>[2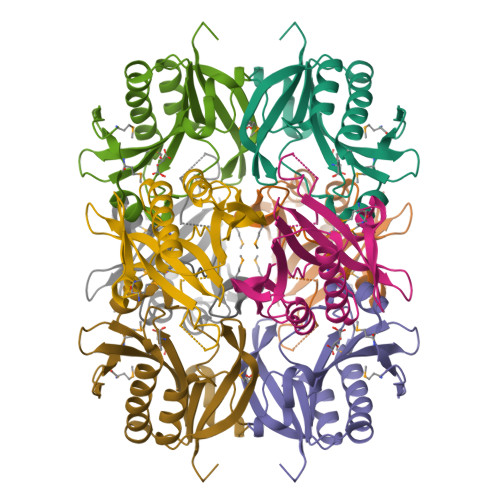x]SNAMQAVYLTGPTVYLRAMVEDDKHHAAAWFDSRFPVNAARAEAFLKEKLQGDPWDARWHLLAIVRRSDEAVVGSCRIEFGKQTASLRFHMAPWLDDADVLRAEALELVVPWLRDEHELLVITVEIAADEQRTLAAAEAAGLKAAVRMREAIARAGHRVDLLIYQAVDPKVEADHA N-[(BENZYLOXY)CARBONYL]-L-ALANINE 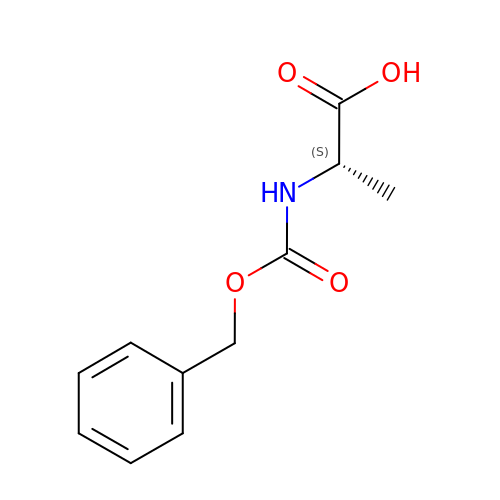| C11 H13 N O4 | TYRGLVWXHJRKMT-QMMMGPOBSA-N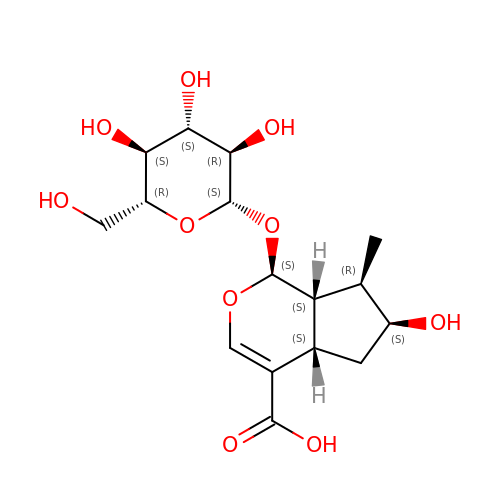Loganic acid | C16 H24 O10 | JNNGEAWILNVFFD-CDJYTOATSA-N>MRRNIFCLACLWIVQACLSLDRADILYNIRQTSRPDVIPTQRDRPVAVSVSLKFINILEVNEITNEVDVVFWQQTTWSDRTLAWNSSHSPDQVSVPISSLWVPDLAAYNAISKPEVLTPQLARVVSDGEVLYMPSIRQRFSCDVSGVDTESGATCRIKIGSWTHHSREISVDPTTENSDDSEYFSQYSRFEILDVTQKKNSVTYSCCPEAYEDVEVSLNFRKKGRSEILGSHHHHHH[10x]

AChBPs are homopentameric, water-soluble homologs of the ligand-binding domain of LGICs and well-established structural surrogates for nicotinic acetylcholine receptors (nAChR). Importantly, AChBPs can bind nAChR-specific ligands and induce similar conformational changes as in the membrane bound receptors. LGICs are activated by ligands binding at subunit interfaces of their extracellular domains, thereby inducing conformational changes that affect the structure of a central pore and its ability to transport ions through the membrane. Additional density was found in all structures at the interface between the subunits in the orthosteric agonist and antagonist binding site, next to loop C in which the respective ligands could be modelled.

In total, five structures of Ls-AChBP in complex with a ligand were successfully solved. The unit cell was comprised of two or four pentamers of Ls-AChBP in the presence of FL1613, FL1856, FL1888, FL3044, VUF24234 and VUF6105. However, the number of binding sites in which additional electron density was observed varied. The electron density in the binding site region was generally poor, indicating that compounds may have had several binding modes in the site. A computational alignment and superimposition of AChBP taken from the protein–ligand complexes and the apo structure showed that there were no large global conformational changes in any of the structures upon ligand binding. However, there were small changes in the loop C region of the crystal structures of Ls-AChBP. When comparing the protomers in complex with a ligand we observed that loop C moves differently upon binding of different compounds. Notably, binding of FL1888, VUF24234 and VUF6105 results in a movement of the loop closer to the compound, while binding of FL1856, FL3044, FL1613 and FL1909 does not have the same effect. The plot indicates that binding of nicotine, FL1613, FL1909, FL1856 and FL3044 do not result in any significant conformational changes in this region, while binding of FL1888, VUF24234 and VUF6105 do.>MAQAKHKQRKRLKSSCKRHPLYVDFSDVGWNDWIVAPPGYHAFYCHGECPFPLADHLNSTNHAIVQTLVNSVNSKIPKACCVPTELSAISMLYLDENEKVVLKNYQDMVVEGCGCR[2x];>[2x]GSGAMAQNLDSMLHGTG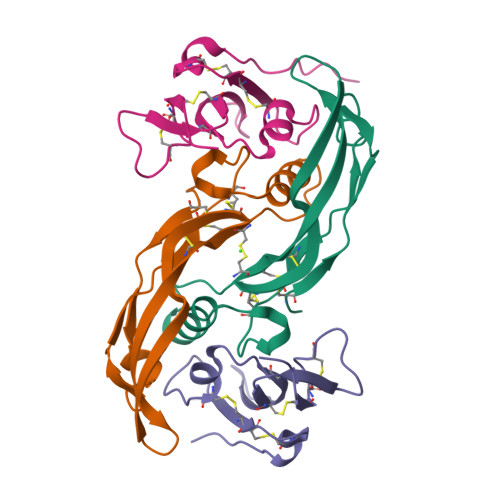MKSDSDQKKSENGVTLAPEDTLPFLKCYCSHHCPEDAINNTCITNGHCFTMIEEDDQGETTLTSGCLGLEGSDFQCRDTPIPHQRRSIECCRTNLCNQYLQPTLPPVVIGPFFDGSIR> GPLGS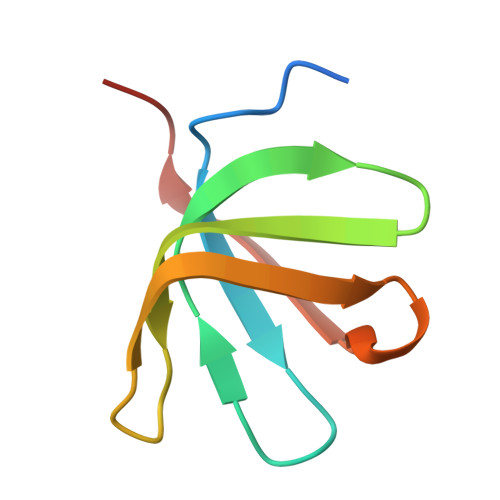MSQFVGFGVQVELKDGKLIQGKIAKATSKGLTLNDVQFGDGGKSQAFKVRASRLKDLKVLTVASQS>MSQYSIQQSLGNASGVAVSPINADATLSTGVALNSSLWAGIGVFARGKPFTVLAVTESNYEDVLGEPLKPSSGSQFEPIRHVYEAIQQTSGYVVRAVPDDAKFPIIMFDESGEPAYSALPYGSEIELDSGEAFAIYVDDGDPCISPTRELTIETATADSAGNERFLLKLTQTTSLGVVTTLETHTVSLAEEAKDDMGRLCYLPTALEARSKYLRAVVNEELISTAKVTNKKSLAFTGGTNGDQSKISTAAYLRAVKVLNNAPYMYTAVLGLGCYDNAAITALGKICADRLIDGFFDVKPTLTYAEALPAVEDTGLLGTDYVSCSVYHYPFSCKDKWTQSRVVFGLSGVAYAAKARGVKKNSDVGGWHYSPAGEERAVIARASIQPLYPEDTPDEEAMVKGRLNKVSVGTSGQMIIDDALTCCTQDNYLHFQHVPSLMNAISRFFVQLARQMKHSPDGITAAGLTKGMTKLL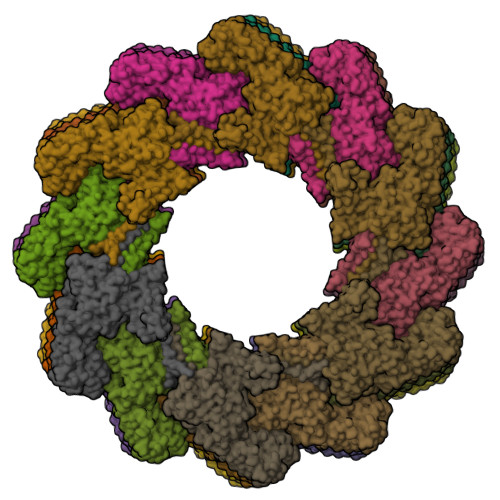DRFVASGALVAPRDPDADGTEPYVLKVTQAEFDKWEVVWACCPTGVARRIQGVPLLIK[30x]> TPPLKSGFVTLQVKNNTNGQYSNDQIYWAIVGKDPDTKQFVHVDLNGNLIPMKISDNDAAGHLTKTTPDGTFNYSNYFCKASQQSYAYIPKIIGARMYISYGKPLYIKVNQAADGLIGYAGPNLANTSDPNT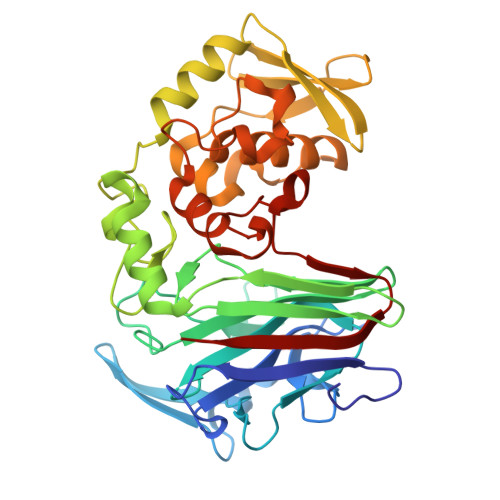GIMFEWAEMAWTNDGLWINTTRVDQFCYPYNIQLVGNSGYNKTYGDTGTRADLMNAYKNSVPAEFKSLVHSDRIYAPASGLGTFTASQANAHYFDSYINDVYSYYATHELTFTCDRGTYSGHVVGNDFVFNKNGGAYNLYIHGKPSTQEVLLGNGIFDGGNDDEKAIKAQVCAAFNRHVMLDPAHWNNSAYFYKDAPANYFAKFWHDHSYENKSYGFCYDDVFDFSSTLHVADPKYAIINVGW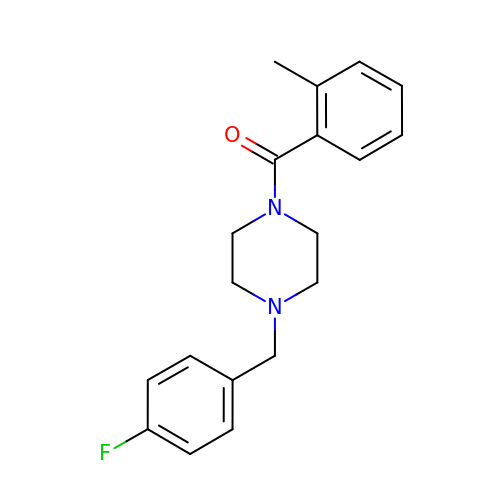[4-[(4-fluorophenyl)methyl]piperazin-1-yl]-(2-methylphenyl)methanone | C19 H21 F N2 O | UONQPTDUVPPQHY-UHFFFAOYSA-N N-[(1S,2R)-1-benzyl-3-(cyclohexylamino)-2-hydroxypropyl]-3-(ethylamino)-5-(2-oxopyrrolidin-1-yl)benzamide | C29 H40 N4 O3 | 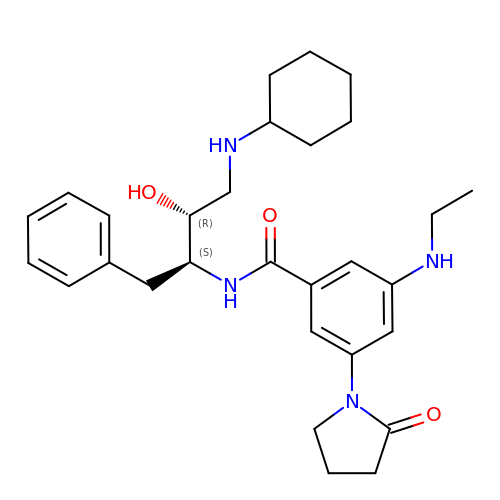PVDHVIVUNLQJLY-RRPNLBNLSA-N>[4x]GSHMSSPSDGPFPKATPQLPNSVFDMFSMKGKVTAITGGGGGIGFAAAEAIAEAGGDVALLYRSAPNMEERSAELAKRFGVKVKSYQCEVTEHESVKQAIEAVEKDFGRLDCYIANAGGGVPGSINPDYPLEAWHKTQSVNLHSTFYAARECARIFKAQGSGSFIATTSISARIVNVPYDQPAYNSSKAAVVHFCRSLARDWRNFARVNTISPGFFDTPMGPSDKAVEDVLYQKSVLGRAGDVKELKAAYLYLASNASTYTTGADLLIDGGYCLT

Recently, for the production of (R)-3-quinuclidinol, 3-quinuclidinone reductase (RrQR) was isolated from Rhodotorula rubra. The purified enzyme from R. rubra is specific to NADPH as a coenzyme and stereospecifically produces the (R)-enantiomer of 3-quinuclidinol from 3-quinuclidinone. Based on the amino acid similarity, RrQR belongs to the short-chain dehydrogenase/reductase family. Therefore, RrQR possesses a novel mechanism for the stereospecific reaction led by a characteristic interaction, in which the hydrophobicity of I167 and F212 plays a crucial role in the stereospecific reduction of 3-quinuclidinone.

The crystal structure of RrQR was determined at 2.2-Å resolution and refined to a crystallographic R-factor of 0.192 and Rfree of 0.230. The asymmetric unit of the crystal contains four protomers of RrQR. A clear electron density for NADPH is observed in each protomer, and the structures of the four NADPH molecules in the asymmetric unit exhibit similar conformations. The crystal structure of RrQR shows a tightly associated homotetramer. Like other SDR family proteins, the RrQR protomer can be divided into two domains: the core and small lobe structures. The NADPH cofactor is located at the bottom of the cleft. The bound NADPH is in an extended conformation, and the nicotinamide and adenine rings are about 10.5 Å apart. Among these residues, R60 and S61 form hydrogen bonds with the 2′-phosphate group of the NADPH; these bonds are involved in the discrimination of NADPH from NADH. In this reductase, residues N138, S166, Y181, and K185 correspond to the catalytic tetrad. A small space is found above the B-face of the nicotinamide ring, and is assumed to be the substrate-binding site. This small pocket, with a diameter of 7 Å and a depth of 8 Å, is formed by S166, I167, S168, N173, Q178, Y181, and F212.>[4x]MARFEEQKLYIGGRYVEASSGATFETINPANGEVLAKVQRASREDVERAVQSAVEGQKVWAAMTAMQRSRILRRAVDILRERNDELAALETLDTGKPLAETRSVDIVTGADVLEYYAGLVPA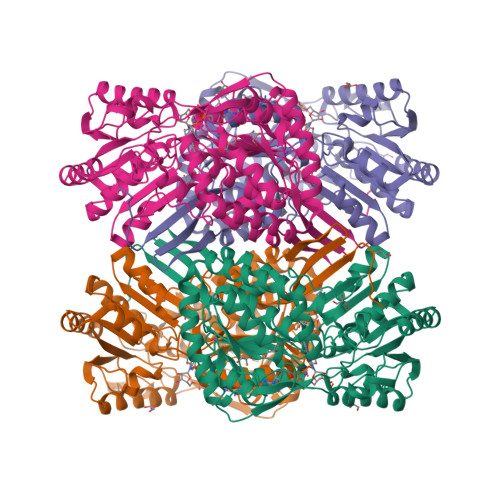IEGEQIPLRETSFVYTRREPLGVVAGIGAWNYPVQIALWKSAPALAAGNAMIFKPSEVTPLTALKLAEIYTEAGVPDGVFNVLTGSGREVGQWLTEHPLIEKISFTGGTSTGKKVMASASSSSLKEVTMELGGKSPLIIFPDADLDRAADIAVMANFFSSGQVATNGTRVFIHRSQQARFEAKVLERVQRIRLGDPQDENTNFGPLVSFPHMESVLGYIESGKAQKARLLCGGERVTDGAFGKGAYVAPTVFTDCRDDMTIVREEIFGPVMSILVYDDEDEAIRRANDTEYGLAAGVVTQDLARAHRAIHRLEAGICWINTWGESPAEMPVGGYKQSGVGRENGLTTLAHYTRIKSVQVELGDYASVF2-{4'-[AMINO(IMINO)METHYL]BIPHENYL-3-YL}-1H-BENZIMIDAZOLE-6-CARBOXIMIDAMIDE 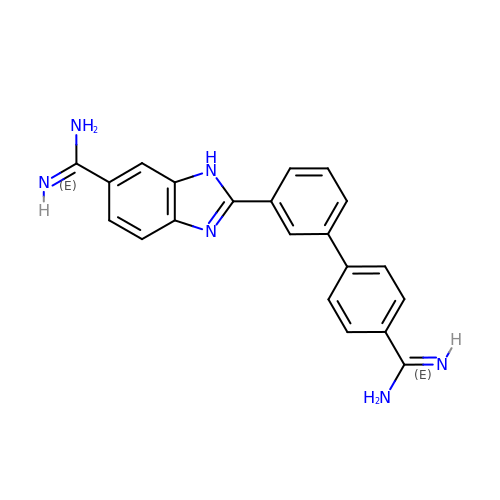| C21 H18 N6 | LRMPNDUSMWYCMH-UHFFFAOYSA-N>MAHHHHHHAALRQPQVAELLAEARRAFREEFGAEPELAVSAPGRVNLIGEHTDYNQGLVLPMALELMTVLVGSPRKDGLVSLLTTSEGADEPQRLQFPLPTAQRSLEPGTPRWANYVKGVIQYYPAAPLPGFSAVVVSSVPLGGGLSSSASLEVATYTFLQQLCPDSGTIAARAQVCQQAEHSFAGMPCGIMDQFISLMGQKGHALLIDCRSLETSLVPLSDPKLAVLITNSNVRHSLASSEYPVRRRQCEEVARALGAASLREVQLEELEAARDLV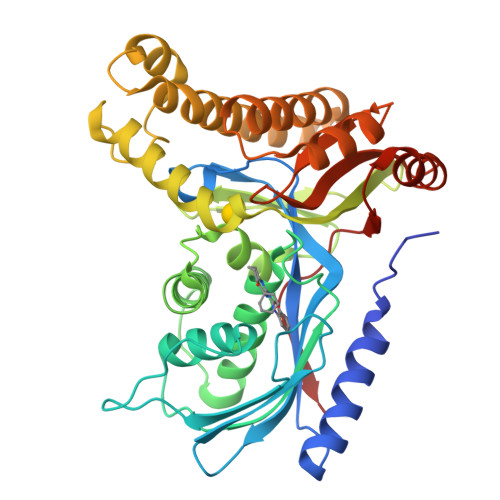SKEGFRRARHVVGEIRRTAQAAAALRRGDYRAFGRLMVESHRSLRDDYEVSCPELDQLVEAALAVPGVYGSRMTGGGFGGCTVTLLEASAAPHAMRHIQEHYGGTATFYLSQAADGAKVLCL[4x]> MELPGALQLGELAAAFASVPVFPLFDAAYFIVSVLYLKYEPGAVEMSRKSPFASWLCAMLHCFGSYILADLLLGESPIHYFSNNSSVILATAV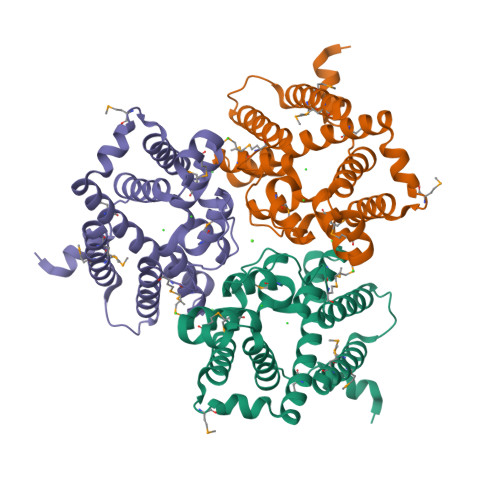WYLIFFCPMNLFYKCVSFLPVKLIFVAMKEVVRVRKIAAGVHHAHHQYHHGWFIMMATGWVKGSGVALMSNFEQLLRGVWRPETNEILHMSFPTKASLYGTVLFTLQQTHWLPVSEANLVFFFTMFMIVCKVFMTATHSHASPFAPVEGFISPVFFGSVSSGHTSHHNQHGHSHEASYQPPPPVKSKEELNEGTRKRKAKKAEAAAENLYFQGLEDYKDDDDKHHHHHHHHHH>GIGTGFPFDPHYVEVLGERMHYVDVGPRDGTPVLFLHGNPTSSYVWRNIIPHVAPTHRCIAPDLIGMGKSDKPDLGYFFDDHVRFMDAFIEALGLEEVVLVIHDWGSALGFHWAKRNPERVKGIAFMEFIRPIPTWDEWPEFARETFQAFRTTDVGRKLIIDQNVFIEGTLPMGVVRPLTEVEMDHYREPFLNPVDREPLWRFPNELPIAGEPANIVALVEEYMDWLHQSPVPKLLFWGTPGVLIPPAEAARLAKSLPNCKAVDIGPGLNLL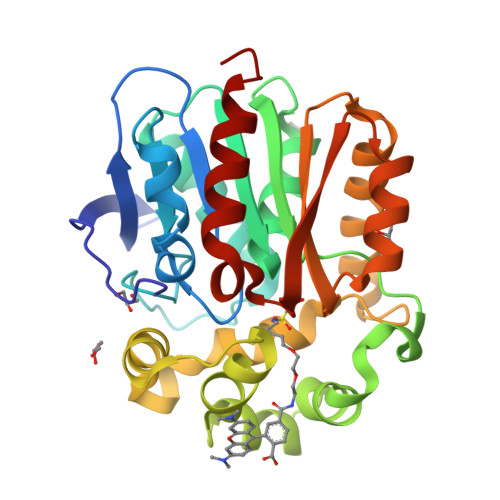QEDNPDLIGSEIARWLSTLEI[2x]> SNISRQAYADMFGPTVGDKVRLADTELWIEVEDDLTTYGEEVKFGGGKVIRDGMGQGQMLAADCVDLVLTNALIVDHWGIVKADIGVKDGRIFAIGKAGNPDIQPNVTIPIGAATEVIAAEGKIVTAGGIDTHIHWICPQQAEEALVSGVTTMVGGGTGPAAGTHATTCTPGPWYISRMLQAADSLPVNIGLLGKGNVSQPDALREQVAAGVIGLKIHEDWGATPAAIDCALTVADEMDIQVALHSDTLNESGFVEDTLAAIGGRTIHTFHTEGAGGGHAPDIITACAHPNILPSSTNPTLPYTLNTIDEHLDMLMVCHHLDPDIAEDVAFAESRIRRETIAAEDVLHDLGAFSLTSSDSQAMGRVGEVILRTWQVAHRMKVQRGALAEETGDNDNFRVKRYIAKYTINPALTHGIAHEVGSIEVGKLADLVVWSPAFFGVKPATVIKGGMIAIAPMGDINASIPTPQPVHYRPMFGALGSARHHCRLTFLSQAAAANGVAERLNLRSAIAVVKGCRTVQKADMVHNSLQPNITVDAQTYEV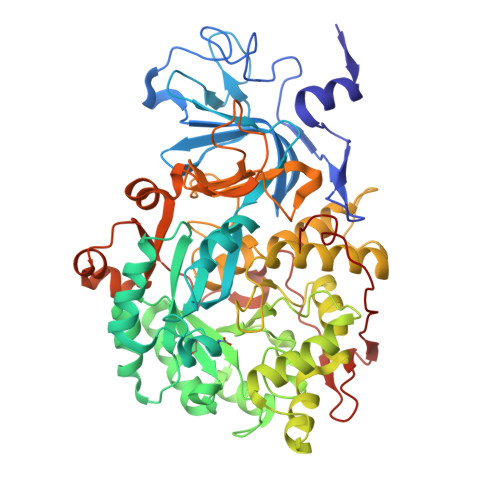RVDGELITSEPADVLPMAQRYFLF5-{5-[1-(pyrrolidin-1-yl)cyclohexyl]-1,3-thiazol-2-yl}-1-{[(2S)-pyrrolidin-2-yl]methyl}-1H-indole | C26 H34 N4 S 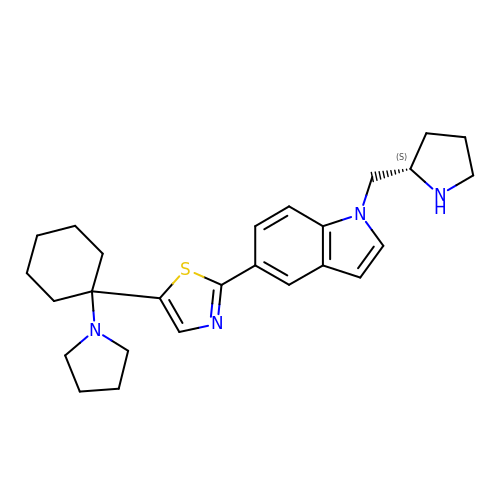| QJVRHGDUROHLPF-QFIPXVFZSA-N> MLLEAIAIALTAAHFGAPLLYYWRAKRWLKKPWDVAPDPTYRPR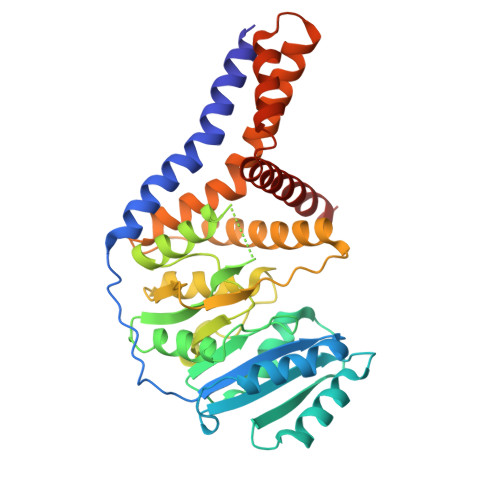VTVIVPTYNEAPLIEEKLDNIYEQDYPRDKLEVVVVDSASTDGTPSAVRRWAETHPDLALTLVEETERRGKAHALNTALRHATGEIVVITDADALWPARDTLANAVKWLADPTVGAVSCVKRPAGPAGVEDSYRDFYNVLRVAESKAWATPIFHGELAAFKRELLERLGGFPTDVGADDSHTATKIAMMGYRAITPPDVVCVEAVPKRGYHAWRIRRAQHLVQHFAKAIRDGKAPPPFKPILHAEAYLHLANPWALPTAAAALAAAAAAGSLPAAALLATGAALALYKPYRTWTTMQAYLIAAAVKNLWDKE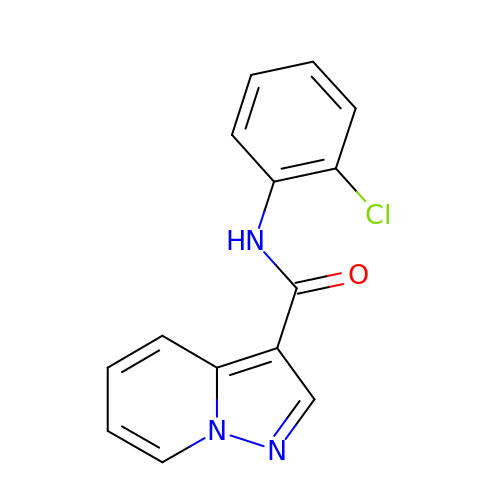N-(2-chlorophenyl)pyrazolo[1,5-a]pyridine-3-carboxamide | C14 H10 Cl N3 O | CPQRFZBWMKEHSA-UHFFFAOYSA-N>SSSSTAAASAKKILVKHVTVIGGGLMGAGIAQVAAATGHTVVLVDQTEDILAKSKKGIEESLRKVAKKKFAENPKAGDEFVEKTLSSISTSTDAASVVHSTDLVVEAIVENLKVKSELFKRLDKFAAEHTIFASNTSSLQITSLANATTRQDRFAGLHFFNPVPLMKLVEVVKTPMTSQKTLESLVDFSKTLGKHPVSCKDTPGFIVNRLLVPYLIEAVRLYERGDASKEDIDTAMKLGAGYPMGPFELLDYVGLDTTKFIIDGWHEMDS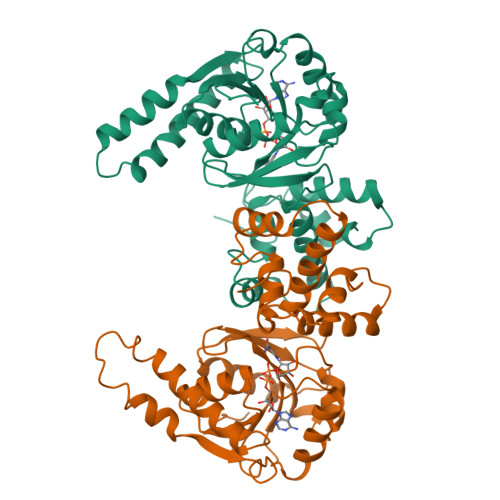QNPLFQPSPAMNKLVAENKFGKKTGEGFYKYK[3x]> GSHVFKSRLQEYAQKYKLPTPVYEIVKEGPSHKSLFQSTVILDGVRYNSLPGFFNRK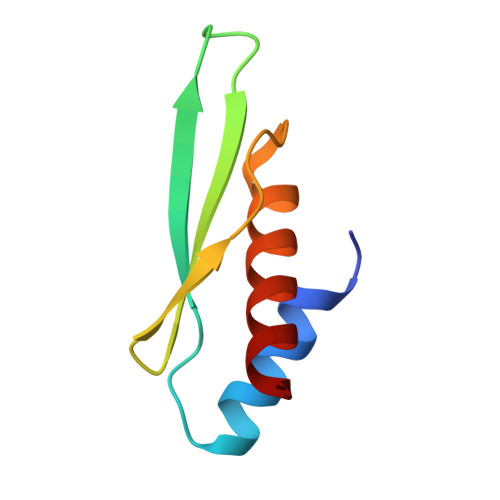AAEQSAAEVALRELAK>[2x]MGSSHHHHHHSSGLVPRGSFQASMKHNINDNTLEIVVGDITKETTNVIVNAANGSLLGGGGVDGAIHHAAGPELLKACQEMRNNELNGEELPTGEVIITSGFQLPSRFIIHTVGPIWNQTPDLQEELLANCYRNALELVKVKKLSSISFPSISTGVYGYPIHEAAAIALQTIIQFLQENDVGLVKVVLFSERDYSIYQEKLKYLIEKI

Macrodomains are ubiquitous and evolutionarily conserved modules (approx. 130–190 residues) that recognize ADPr derivatives in their free form or linked to proteins, including ADPr, PAR, ADP-ribose-1″phosphate and O-acetyl-ADPr (OAADPr). To expand our knowledge concerning the field of macrodomains, we have characterized Oceanobacillus iheyensis macrodomain (OiMacroD), the first to be described from the order Bacillales. A yield of 40 mg of pure protein per litre of culture after a simple two-step purification process was obtained. Its phylogenetic analysis revealed that, among the six different classes previously described for macrodomains, OiMacroD is included in the MacroD-type clade, together with other previously characterized MacroD-like macrodomains, such as hMacroD1 and hMacroD2. The subunit has a mixed α/β fold, similar to that of other nucleotide-binding proteins, composed of a central seven-stranded mixed β-sheet (β1–β2–β7–β6–β3–β5–β4) and five α-helices.

Three crystal structures of monomeric OiMacroD wild-type (WT) complexed with MES, ADPr or ADP were obtained at 1.9, 1.77 and 1.75 Å resolution, respectively. The best WT and G37V crystals were grown in 0.2 M ammonium sulphate, 0.1 M MES pH 6.5 and 30% (w/v) PEGMME 5 K. D40A and N30A mutant crystals were grown in 0.2 M magnesium formate with 20% (w/v) PEG3350 or 20% (w/v) PEG1500 with 20% glycerol, respectively. Of note is the finding of a set of five well-ordered water molecules (W1–W5) fixed in the active centre of OiMacroD. The presence of these water molecules represents a constant, previously undescribed element in the macrodomain binding site of Bacteria, Archaea and Eukarya, even in the absence of ligands. A precise H-bond network for adenosine moiety binding was found in both the presence and absence of ligand, consisting of three fixed conserved water molecules (W1–W3).> MSLAPGKAE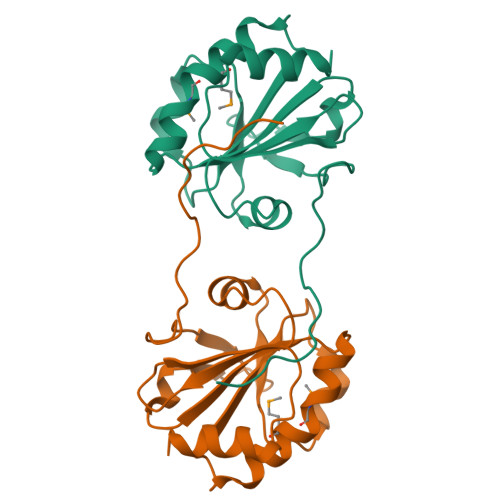SDAPLVRTGALAPNFKLPTLSGENKSLAQYRGKIVLVNFWASWCPYCRDEMPSMDRLVKSFPKGDLVVLAVNVEKRFPEKYRRAPVSFNFLSDATGQVQQRYGANRLPDTFIVDRKGIIRQRVTGGIEWDAPKVVSYLKSLEGHHHHHH>[2x]MGSSHHHHHHSSPRLFMLSSTSSDALRQTARQLATWVEEHQDCVAASDLAYTLARGRAHRPVRTAVVAANLPELVEGLREVADGDALYDAAVGHGDRGPVW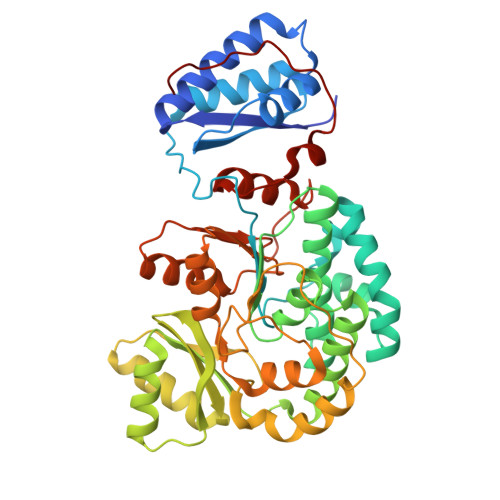VFSGQGSQWAAMGTQLLASEPVFAATIAKLEPVIAAESGFSVTEAITAQQTVTGIDKVQPAVFAVQVALAATMEQTYGVRPGAVVGHSVGESAAAVVAGALSLEDAARVICRRSKLMTRIAGAGAMGSVELPAKQVNSELMARGIDDVVVSVVASPQSTVIGGTSDTVRDLIARWEQRDVMAREVAVDVAFHSPQVDPILDDLAAALADIAPMTPKVPYYSATLFDPREQPVCDGAYWVDNLRNTVQFAAAVQAAMEDGYRVFAELSPHPLLTHAVEQTGRSLDMSVAALAGMRREQPLPHGLRGLLTELHRAGAALDYSALYPAGRLVDAPLPAWGS> MAYTSHLSSKTGLHFGRLSLRSLTAYAPNLMLWGGASMLGLFVFTEG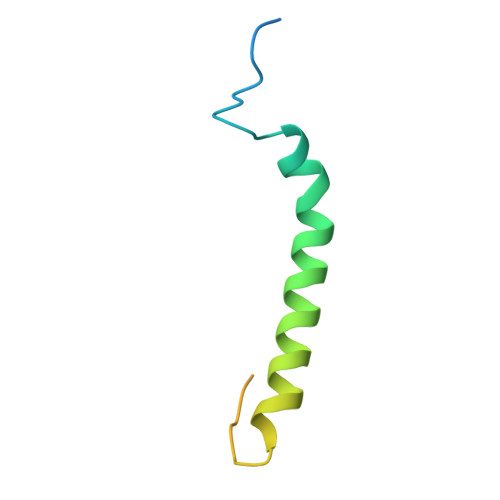WPKFQDTLYKKIPLLGPTLEDHTPPEDKPN>GAGEGQGPKKQTRLGLEAKKEENLADWYSQVITKSEMIEYHDISGCYILRPWAYAIWEAIKDFFDAEIKKLGVENCYFPMFVSQSALEKEKTHVADFAPEVAWVTRSGKTELAEPIAIRPTSETVMYPAYAKWVQSHRDLPIKLNQWCNVVRWEFKHPQPFLRTREFLWQEGHSAFATMEEAAEEVLQILDLYAQVYEELLAIPVVKGRKTEKEKFAGGDYTTTIEAFISASGRAIQGGTSHHLGQNFSKMFEIVFEDPKIPGEKQFAYQNSWGLTTRTIGVMTMVHGDNMGLVLPPRVACVQVVIIPCGITNALSEEDKEALIAKCNDYRRRLLSVNIRVRADLRDNYSPGWKFNHWELKGVPIRLEVGPRDMKSCQFVAVRRDTGEKLTVAENEAETKLQAILEDIQVTLFTRASEDLKTHMVVANTMEDFQKILDSGKIVQIPFCGEIDCEDWIKKTTARDQDLEPGAPSMGAKSLCIPFKPLCELQPGAKCVCGKNPAKYYTLFGRSY[2x]

Human cytosolic prolyl-tRNA synthetase (HcProRS) catalyses the formation of the prolyl-tRNAPro, playing an important role in protein synthesis. Notably, glutamyl-prolyl-tRNA synthetase (EPRS) is a dual function enzyme that catalyses the formation of charged glutamyl-tRNA and prolyl-tRNA in the cytoplasm. The human ProRS (HcProRS) activity is located at the C-terminal region of this protein and inhibition of this enzyme has been recognized as a promising approach for treatment of HcProRS-related diseases. Inhibition of HcProRS activity has been shown to have potential benefits in the treatment of fibrosis, autoimmune diseases and cancer.

To further clarify the binding mechanism of the identified hits, we determined five co-crystal structures of HcProRS in complex with the corresponding compound and Pro at a resolution range of 2.2–2.7 Å. In the presence of the natural substrate Pro, the Tm of HcProRS increased by 4 °C. Normalized by this control, the presence of five of the 17 compounds, including 4h (R = 2-Cl) and 4j (R = 2-CF3), significantly improved the thermal stability of HcProRS resulting with ∆Tm values in a range of 2 to 7 °C suggesting these compounds are likely binding to HcProRS in a Pro-dependent manner. The EC50 values of 4h (R = 2-Cl) and 4j (R = 2-CF3) proved 6-fold better than R = 2-CH3 in compound 4d, indicating that the electron withdrawing properties might be beneficial for binding. Similar phenomenon was also observed for the 3.6-fold lower EC50 of double substituted compound 3b (R = 2-Cl) when compared with the single substituted 4h. Combined, the positive electrostatic potential of this binding pocket indicated that an electronegative substituent at ortho-position of the C3-amine benzyl ring is likely better than neutral or electron-deficient substituents. This is evidenced by the 7-fold better binding potency of 2-Cl and 2-CF3 substituted compound 4h and 4j compared with 2-CH3 substituted 4d and 2-fold lower EC50 of 3b (2-Cl) relative to 3c (2-CH3). However, in our ligand-bound structures, no electron density of equivalent water is observed, and the ortho-substituents (2-Cl, 2-CF3 and 2-CH3) of our compounds seem to replace this structured water. The similar stabilization of the benzyl ring was also detected for the other studied 2-substituted compounds 4d and 4h.> MSA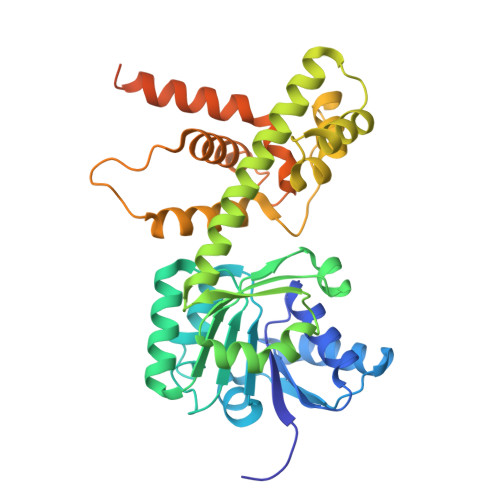IKRSLNVGVVGMGNMGVPIARNLGFKARSAMYLQIHSRALSKAKRVCDDLSVDGATCAMRIHDRYSTMTKWCDVIVLALADVKASRHALLEDNESLIMNARKGQIIVDHTTVDAETSRECAHEAARRGAYFLDAPMSGSPRACFNGQLLLMVGGDAETFQKMLPIFHMYADNVFHMGESGSGTAAKMISQALVASHNAAAAEALSMAHALGIEDQSKLVQVLDASWGSSTMLRRNAPLLQDLIRNPDKTPPTSAVSVDRLLSDLAHLDASLPKRGGEDEPFPVFDAALRSLAAASDAGMGDRDLASVVHYIEAGEAELRNRTHVPLXGEHLTGRTAATAANSSVNETPSTVNGSSEVPNEFGVEDFY>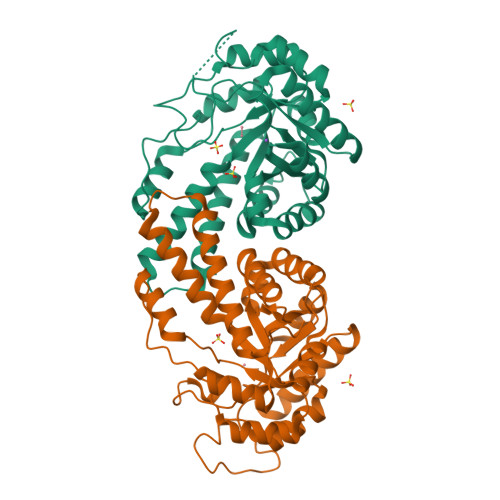[4x]MLVTGLEILKKAREEGYGVGAFNVNNMEFLQAVLEAAEEQRSPVILALSEGAMKYGGRALTLMAVELAKEARVPVAVHLDHGSSYESVLRALRAGFTSVMIDKSHEDFETNVRETRRVVEAAHAVGVTVEAELGRLAGIEEHVAVDEKDALLTNPEEARIFMERTGADYLAVAIGTSHGAYKGKGRPFIDHARLERIARLVPAPLVLHGASAVPPELVERFRASGGEIGEAAGIHPEDIKKAISLGIAKINTDTDLRLAFTALIREALNKNPKEFDPRKYLGPAREAVKEVVKSRMELFGSVGRA> MSEMSLIMLAAGNSTRFNTKVKKQFLRLGNDPLWLYATKNLSSFYPFKKIVVTSSNITYMKKFTKNYEFIEGGDTRAESLKKALELIDSEFVMVSDVARVLVSKNLFDRLIENLDKADCITPALKVADTTLFDNEALQREKIKLIQTPQISKTKLLKKALDQNLEFTDDSTAIAAMGGKIWFVEG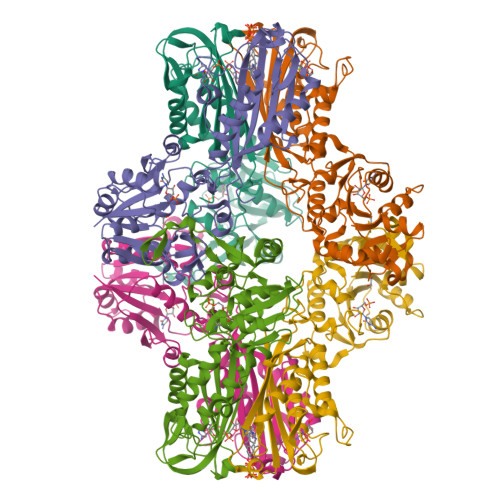EENARKLTFKEDLKKLDLPTPSFEIFTGNGFDVHEFGENRPLLLAGVQIHPTMGLKAHSDGDVLAHSLTDAILGAAGLGDIGELYPDTDMKFKNANSMELLKQAYDKVREIGFELINIDICVMAQSPKLKDFKQAMQSNIAHTLDLDEFRINVKATTTEKLGFIGRKEGMAVLSSVNLKYFDWTRL1-DEOXY-1-THIO-HEPTAETHYLENE GLYCOL | C14 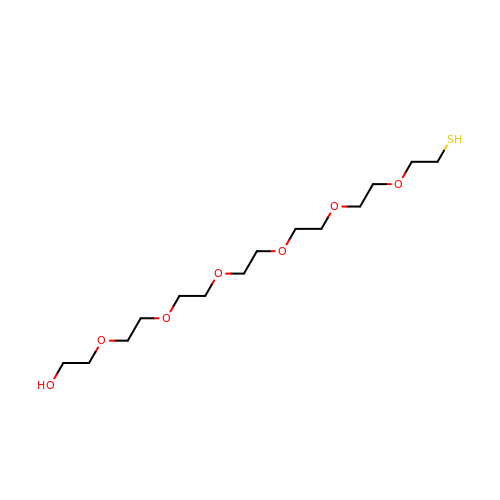H30 O7 S | ACMBXVJDKVNCGH-UHFFFAOYSA-N>MAAACRSVKGLVAVITGGASGLGLATAERLVGQGASAVLLDLPNSGGEAQAKKLGNNCVFAPADVTSEKDVQTALALAKGKFGRVDVAVNCAGIAVASKTYNLKKGQTHTLEDFQRVLDVNLMGTFNVIRLVAGEMGQNEPDQGGQRGVIINTASVAAFEGQVGQAAYSASKGGIVGMTLPIARDLAPIGIRVMTIAPGLFGTPLLTSLPEKVCNFLASQVPFPSRLGDPAEYAHLVQAIIENPFLNGEVIRLDGAIRMQP[4x];> SRPRKDPLRHLRTREKRGPSGCSGGPNTVYLQVVAAGSRDSGAALYVFSEFNRYLFNCGEGVQRLMQEHKLKVARLDNIFLTRMHWSNVGGLSGMILTLKETGLPKCVLSGPPQLEKYLEAIKIFSGPLKGIELAVRPHSAPEYEDETMTVYQIPIHSEQRRGKHQPWQSPERPLSRLSPERSSDSESNENEPHLPHGVSQRRGVRDSSLVVAFICKLHLKRGNFLVLKAKEMGLPVGTAAIAPIIAAVKDGKSITHEGREILAEELCTPPDPGAAFVVVECPDESFIQPICENATFQRYQGKADAPVALVVHMAPASVLVDSRYQQWMERFGPDTQHLVLNENCASVHNLRSHKIQTQLNLIHPDIFPLLTSFRCKKEGPTLSVPMVQGECLLKYQLRPRREWQRDAIITCNPEEFIVEALQLPNFQQSVQEYRRSAQDGPAPAEKRSQYPEIIFLGTGSAIPMKIRNVSATLVNISPDTSLLLDCGEGTFGQLCRHYGDQVDRVLGTLAAVFVSHLAADHHTGLPSILLQRERALASLGKPLHPLLVVAPNQLKAWLQQYHNQCQEVLHHISMIPAKCLQEGAEISSPAVERLISSLLRTCDLEEFQTCLVRHCKHAFGCALVHTSGWKVVYSGDTMPCEALVRMGKDATLLIHEATLEDGLEEEAVEKTHSTTSQAISVGMRMNAEFIMLNHFSQRYAKVPLFSPNFSEKVGVAFDHMKVCFGDFPTMPKLIPPLKALFAGDIEEMEERREKRELRQVRAALLSRELAGGLEDGEPQQKRAHTEEPQAKKVRAQ;> MKSSVQEECVSTISSSKDEDPLAATREFIEMWRLLGREVPEHITEEELKTLMECVSNTAKKKYLKYLYTKEKVKKARQIKKEMKAAAREEAKNIKLLETTEEDKQKNFLFLRLWDRNMDIAMGWKGAQAMQFGQPLVFDMAYENYMKRKELQNTVSQLLESEGWNRRNVDPFHIYFCNLKIDGALHRELVKRYQEKWDKLLLTSTEKSHVDLFPKDSIIYLTADSPNVMTTFRHDKVYVIGSFVDKSMQPGTSLAKAKRLNLATECLPLDKYLQWEIGNKNLTLDQMIRILLCLKNNGNWQEALQFVPKRKHTGFLEISQHSQEFINRLKKAKTAENLYFQSHHHHHHDYKDDDDK

Here, we present several cryo-EM structures of the mitochondrial RNase Z complex (ELAC2/SDR5C1/TRMT10C) bound to different maturation states of mitochondrial tRNAHis, showing the molecular basis for tRNA-substrate selection and catalysis. The human long form of RNase Z, ELAC2, has two alternative start codons to produce a nuclear and a mitochondrially targeted form. TRMT10C is a purine N1-methyltransferase that acts at position 9 of mt-tRNAs using S-adenosylmethionine (SAM) as a co-substrate. SDR5C1 is a moonlighting homotetrameric short-chain dehydrogenase/reductase.

To trap an mt-RNase Z substrate-relevant complex, we mutated H548, which coordinates one of the two active site Zn2+ ions and determined a 2.9 Å resolution cryo-EM structure from a mitochondrial RNase Z (H548A) complex preparation in which the mt-tRNA precursor was predominantly uncleaved (RNase ZH548A-HS). Overall, the structure of the TRMT10C/SDR5C1/mt-tRNA platform did not change with the introduction of the H548A mutation. However, ELAC2 pivots on the mt-tRNA by approximately 3.5° (Fig. EV3A) compared with its position in the product complex. Due to this pivoting, the RNase ZH548A-HS structure shows a difference in the interactions around the discriminator nucleotide and the scissile bond compared with the product complex. In the RNase ZH548A-HS structure, the 3′-oxygen of the scissile bond is properly oriented for hydrolysis, but it is displaced by ~3 Å, and the discriminator nucleotide C73 moves closer to E130. This may be attributed to the absence of the first Zn2+ ion due to the H548A mutation. Notably, K700 switches from interacting with C72 in the product complex RNase Z-HS to interacting with the scissile bond, i.e., the C73-G1 phosphodiester bond in the RNase ZH548A-HS structure. The scissile bond is followed by the mt-tRNASer(AGY) acceptor stem. Only the first nucleotide (G1) was modeled; nevertheless, the cryo-EM map contains additional density for the mt-tRNASer(AGY) (Figs. 4B and EV3B) and reveals that the acceptor stem contacts ELAC2 residues G156-P157 (Fig. EV3C), which are situated on a ridge in the 3′-direction of the substrate RNA. Taken together, in comparison with the RNase Z-HS product structure, the RNase ZH548A-HS structure reveals additional ELAC2 residues involved in binding to the mt-tRNA precursor and in orienting the scissile bond, namely E130, K700, and G156-P157.>SNAMGLDVRNNGNDNVEIRAAETRTAQRADEALETAADFAGQPKV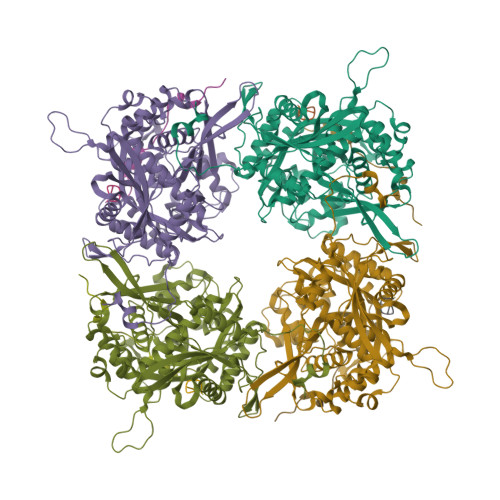THTMRTINRTLSRRISRNTGSEQVLNLRRLMEKYLEDTRFKDDFIFVAVDPNQYSVPYPTLVVMSGAKVGDHNHFFGYVLPLVAGLAPLPRREEQGPHGNILVPRTWVDNLNGTFINEVMAAMYAAIGGKSNGTARIAGLAVVTNEITAESAHLATTLLSAADNAIQTAIEIRLGDKLGLPQFNLGMMASDQPISSVQYNTSGMQDSDIVGNPVRSDITVTISNRIRQAMSDYDSQQRLVATTGYIDLTYSPQNPTFNQGPVLVNGYPVPPTVQYQPRYVMTSAYPLELDAFTPNTFVLGLIGTIATLNSGMAWAQSLISNAARGIGPHNPGALAMVLDPEVTAPLDLSTQTNEQIYKFLQQVLYPSLLISIDVPEEGEYSWLLRMIPAAEKIYTGKVEGEVREISEGYKALYRAFDDVTLGCFSKKYQYGLPLVYATGNRIPLGHYNHQDGHRHDIRDMDDLYMMNITNPDTVEAWEDSFDRTDMTMSQRVVARHEIIDRVLSGSWEQTGWAMRYDFDPLALQALIEAAADAGFTIRPENIQHLAGTAVRGNMAARARGLGNISGNIYARSDRPNVGVNNMGGAFNLF[12x]> MEKDGLCRADQQYECVAEIGEGAYGKVFKARDLKNGGRFVALKRVRVQTGEEGMPLSTIREVAVLRHLETFEHPNVVRLFDVCTVSRTDRETKLTLVFEHVDQDLTTYLDKVPEPGVPTETIKDMMFQLLRGLDFLHSHRVVHRDLKPQNILVTSSGQIKLADFGLARIYSFQMALTSVVVTLWYRAPEVLLQSSYATPVDLWSVGCIFAEMFRRKPLFRGSSDVDQLGKILDVIGLPGEEDWPRDVALPRQAFHSKSAQPIEKFVTDIDELGKDLLLKCLTFNPAKRISAYSALSHPYFQDLERCKENLDSHLPPSQNTSELNTA;> MLLEEVCVGDRLSGAAARGDVQEVRRLLHRELVHPDALNRFGKTALQVMMFGSPAVALELLKQGASPNVQDASGTSPVHDAARTGFLDTLKVLVEHGADVNALDSTGSLPIHLAIR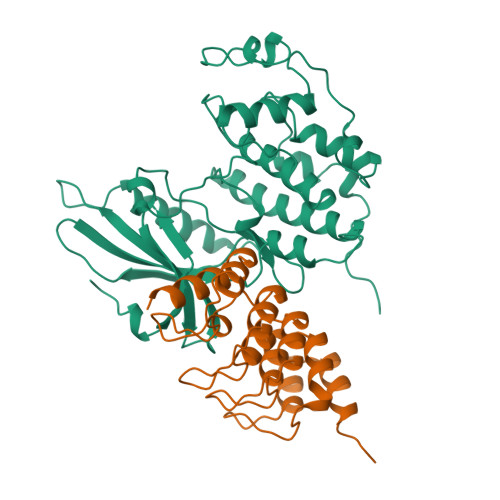EGHSSVVSFLAPESDLHHRDASGLTPLELARQRGAQNLMDILQGHMMIPM GuaB catalyzes the oxidation of the substrate inosine-5´-monophosphate (IMP) to xanthosine 5´-monophosphate (XMP) using NAD+ as a cofactor, and guanosine 5´-monophosphate (GMP) synthase converts XMP to guanosine 5'- monophosphate (GMP) to generate guanine nucleotides essential for cell growth and viability. Indeed, genetic studies have shown that de novo guanine biosynthesis is essential for growth and viability of bacteria both in vitro and in vivo (10–23). Here, we present the first high resolution co-crystal structures of A. baumannii, S. aureus, and E. coli GuaB proteins (cystathionine beta-synthase (CBS) domains deleted), each determined with a matched set of three different inhibitors bound. Similarly, the NAD+ binding region, also where our compounds bind, occurs at the junction between neighboring molecules with side chains from both protomers contributing to ligand binding interactions.

The novel S. aureus and E. coli structures crystallize with one molecule in the asymmetric unit (asu), yet re-create the common GuaB tetramer arrangement via the fourfold symmetry operator of their I4 space group. Common to all three species’ structures, the amino- and carboxy-terminal ends of the protein are engaged in mutually reciprocal strand swaps with their neighboring protomer around the tetramer. We observed a tight overlay of structures across the bacterial strains, highlighting common critical interactions required for potency. These inhibitors mimic the NADH/IMP cofactor interactions by forming strong π-π stacking interactions with IMP while also hydrogen bonding with the conserved glycine (Gly299Ab/302Sa/300Ec) which is one of the two hydrogen bond interactions observed with the NADH amide. The ligand linker segment induces a 90° bend, directing either the amide N-H of G2 and G1 or the imidazole of G8 to form an important hydrogen bond to the conserved glutamic acid (Glu416Ab/417Sa/415Ec) while directing the aryl tail group into a hydrophobic shelf region. Differences in the polarity of a particular key selectivity residue specifically (Ser250 in E. coli versus Ala252 in S. aureus and Ala249 in A. baumannii) was found to be critical for inhibitor interaction with GuaB which corroborates the observations of previous reports. The key residues (SER-440 and SER-250) in the binding site of GuaB E. coli contribute to a stable and extensive water network (more green and well-connected spheres) predicted by WaterMap analysis with the pseudo-apo crystal structures. To disrupt such water network, the compound needs to pay a larger desolvation penalty leading to poor potency, whereas the same compound binding to GuaB in S. aureus and A. baumannii does not need to pay for such penalty with a less favorable water network (more red and less connected spheres).

> MHHHHHHGENLYFQGSWESKFAKESLTFDDVLLIPAQSDILPKDVDLSVQLSDKVKLNIPVISAGMDTVTESKMAIAMARQGGLGVIHKNMGVEEQADEVQKVKRSGGLLVAAAIGISKDTDIRAQKLVEAGVDVLVIDTAHGHSKGVIDQVKHIKKTYPEITLVAGNVATAEATKDLFEAGADIVKVGIGPGSICTTRVVAGVGVPQITAIYDCATEARKHGKAIIADGGIKFSGDIIKALAAGGHAVMLGSLLAGTEESPGATEIFQGRQYKVYRGMGSLGAMEKGSNDRYFQEDKAPKKFVPEGIEGRTAYKGALQDTIYQLMGGVRAGMGYTGSHDLRELREEAQFTRMGPAGLAESHPHNIQITKESPNYSFGNS>GAMDRVPIMYPIGQMHGTYILAQNENGLYIIDQHAAQERIKYEYFREKVGEVEPEVQEMIVPLTFHYSTNEALIIEQHKQELESVGVFLESFGSNSYIVRCHPAWFPKGEEAELIEEIIQQVLDSKNIDIKKLREEAAIMMSCKGSIKANRHLRNDE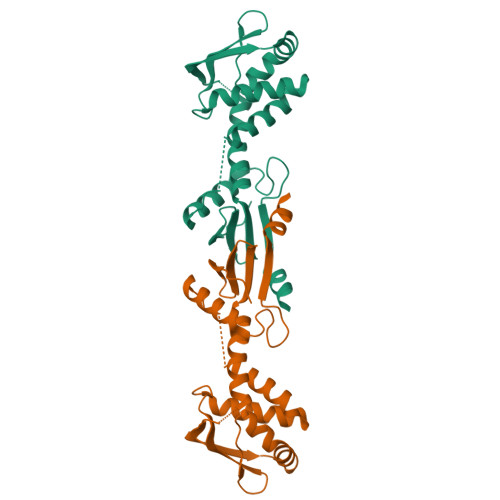IKALLDDLRSTSDPFTCPHGRPIIIHHSTYEMEKMFKRVM[4x]> GGGAEALELLEHCGVCRERLRPEREPRLLPCLHSACSACLGPAAPAAANSSGDGGAAGDGTVVDCPVCKQQCFSKDIVENYFMRDSGSKAGERTVYCNVHKHEPLVLFCESCDTLTCRDCQLNAHKDHQYQFLEDAVRNQRKLLASLVKRLGDKHATLQKSTKEVRSSIRQVSDVQKRVQVDVKMAILQIMKELNKRGRVLVNDAQKVTEGQQERLERQHWTMTKIQKHQEHILRFASWALESDNNTALLLSKKLIYFQLHRALKMIVDPVEPHGEMKFQWDLNAWTKSAEAFGKIVAERPGTNSTGPAPMAPPRAPGPLSK;> LSELEDLKDAKLQTLKELFPQRSDNDLLKLIESTSTMDGAIAAALLMF

SMARCAD1 is a chromatin remodeler, a member of the SWI2/SNF2-like family of enzymes that couple ATP hydrolysis to repositioning, ejecting, or restructuring nucleosomes. KAP1 (also known as TRIM28 and TIF1β) is the major interaction partner of SMARCAD1, with the two proteins forming a tight complex (Okazaki et al., 2008, Rowbotham et al., 2011). The SMARCAD1-KAP1 interaction is direct and involves the first SMARCAD1 CUE domain (CUE1) and the RBCC domain of KAP1. Remarkably, CUE1, a canonical CUE domain, recognizes a cluster of exposed hydrophobic and surrounding charged/amphipathic residues on KAP1, which are presented in the context of a coiled-coil domain, not in a structure resembling ubiquitin.

To improve the diffraction resolution, a KAP1 RBCC construct lacking residues 141–202 (KAP1 RBCC ΔBBX1) was produced. Crystals of the KAP1 RBCC ΔBBX1-SMARCAD1 CUE1,2 complex were tetragonal, and diffracted to 3.7 Å resolution. The structure was solved by molecular replacement using the cubic crystal structure as a search model. Similar to other TRIM family members (Goldstone et al., 2014, Sanchez et al., 2014, Weinert et al., 2015), the biological unit is a single, elongated dimer, which is symmetrical in the tetragonal crystal form (KAP1 RBCC ΔBBX1-SMARCAD1 CUE1,2 complex) but slightly asymmetric in the cubic crystal form (KAP1 RBCC-SMARCAD1 CUE 1,2 complex), suggesting that the coiled-coil domains may have a somewhat dynamic structure. In both cases, the dimer interface is extensive (∼5100 Å2) and formed primarily by the antiparallel association of the coiled-coil domains, with some contributions from the RING and second B-box domains. In both structures, electron density was only observed for a single CUE domain, which we conclude must be SMARCAD1 CUE1 based on our biochemical data. The majority of contacts (i.e., ∼520 Å2 of a total interface area of ∼600 Å2) are between CUE1 and an exposed surface at the C-terminal end of the long arm of the coiled-coil domain of one KAP1 subunit, but the interface also involves the RING domain of the other KAP1 subunit of the homodimer. The α1 helix of SMARCAD1 CUE1 overlies and buries the exposed KAP1 RBCC hydrophobic cluster that is comprised of residues I338, L376, M378, I379, and V380. Thus, CUE1 α1 helix residues such as Q163, T164, E167, and L168 contact the exposed KAP1 RBCC hydrophobic residues, with T164 appearing to be particularly critical. The CUE1 α3 helix—despite containing the conserved di-leucine repeats, L195 and L196—contributes only minimally to the interaction interface via contacts with the peripheral charged/amphipathic KAP1 residues (e.g., R330, W333, and T334).>MLNQELELSLNMAFARAREHRHEFMTVEHLLLALLSNPSAREALEACSVDLVALRQELEAFIEQTTPVLPASEEERDTQPTLSFQRVLQRAVFHVQSSGRNEVTGANVLVAIFSEQESQAAYLLRKHEVSRLDVVNFISHGTRKDEPTQSSDPGSQPNSEEQAGGEERMENFTTNLNQLARVGGIDPLIGREKELERAIQVLCRRRKNNPLLVGESGVGKTAIAEGLAWRIVQGDVPEVMADCTIYSLDIGSLLAGTKYRGDFEKRFKALLKQLEQDTNSILFIDEIHTIIGAGAASGGQVDAANLIKPLLSSGKIRVIGSTTYQEFSNIFEKDRALARRFQKIDITEPSIEETVQIINGLKPKYEAHHDVRYTAKAVRAAVELAVKYINDRHLPDKAIDVIDEAGARARLMPVSKRKKTVNVADIESVVARIARIPEKSVSQSDRDTLKNLGDRLKMLVFGQDKAIEALTEAIKMARAGLGHEHKPVGSFLFAGPTGVGKTEVTVQLSKALGIELLRFDMSEYMERHTVSRLIGAPPGYVGFDQGGLLTDAVIKHPHAVL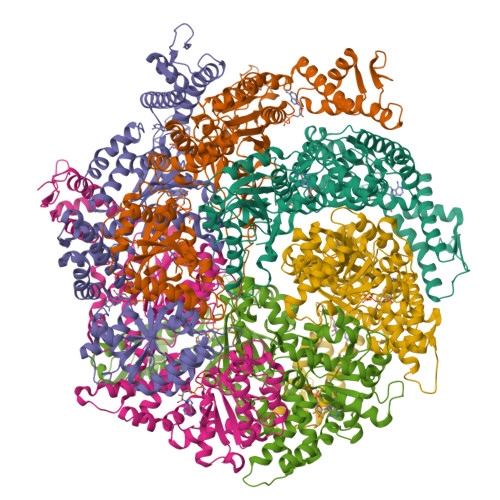LLDEIEKAHPDVFNILLQVMDNGTLTDNNGRKADFRNVVLVMTTNAGVRETERKSIGLIHQDNSTDAMEEIKKIFTPEFRNRLDNIIWFDHLSTDVIHQVVDKFIVELQVQLDQKGVSLEVSQEARNWLAEKGYDRAMGARPMARVIQDNLKKPLANELLFGSLVDGGQVTVALDKEKNELTYGFQSAQKHKAEAAH[6x]> YVDVGPDSVKSACIEVDIQQTFFDKTWPRPIDVS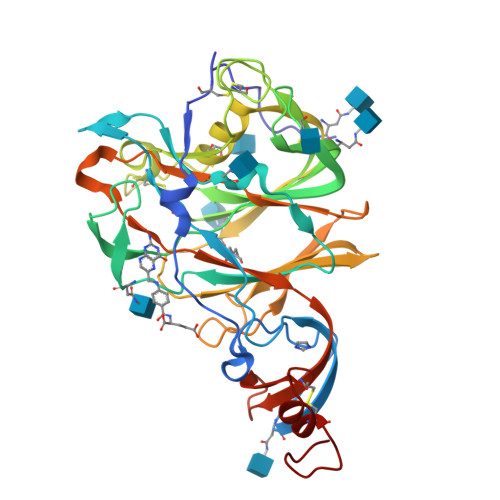KADGIIYPQGRTYSNITITYQGLFPYQGDHGDMYVYSAGHATGTTPQKLFVANYSQDVKQFANGFVVRIGAAANSTGTVIISPSTSATIRKIYPAFMLGSSVGNFSDGKMGRFFNHTLVLLPDGCGTLLRAFYCILEPRSGNHCPAGNSYTSFATYHTPATDCSDGNYNRNASLNSFKEYFNLRNCTFMYTYNITEDEILEWFGITQTAQGVHLFSSRYVDLYGGNMFQFATLPVYDTIKYYSIIPHSIRSIQSDRKAWAAFYVYKLQPLTFLLDFSVDGYIRRAIDCGFNDLSQLHCSYESGLEVLFQ5-(4-CHLORO-PHENYL)-6-ETHYL-PYRIMIDINE-2,4-DIAMINE 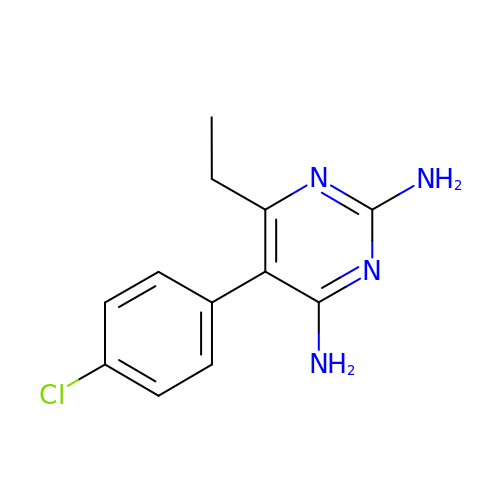| C12 H13 Cl N4 | WKSAUQYGYAYLPV-UHFFFAOYSA-N>[2x]MTAGSDRRPRDPAGRRQAIVEAAERVIARQGLGGLSHRRVAAEANVPVGSTTYYFNDLDALREAALAHAANASADLLAQWRSDLDKDRDLAATLARLTTVYLADQDRYRTLNELYMAAAHR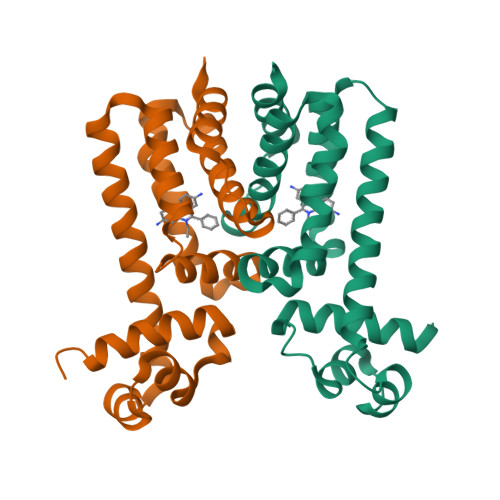PELQRLARLWPDGLLALLEPRIGRRAANAVTVFFDGATLHALITGTPLSTDELTDAIARLVADGPEQREVGQSAHAGRTPDHHHHHH> MNISDVAKITGLTSKAIRFYEEKGLVTPPMRSENGYRTYTQQHLNELTLLRQARQVGFNLEESGELVNLFNDPQRHSADVKRRTLEKVAEIERHIEELQSMRDQLLALANACP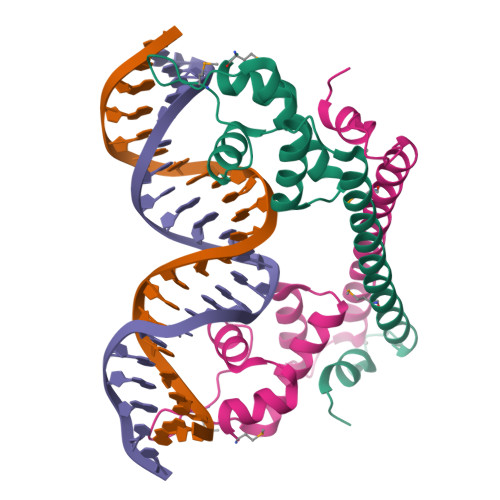GDDSADCPIIENLSGCCHHRAG> MAARWSSENVVVEFRDSQATAMSVDCLGQHAVLSGRRFLYIVNLDAPFEGHRKISRQSKWDIGAVQWNPHDSFAHYFAASSNQRVDLYKWKDGSGEVGTTLQGHTRVISDLDWAVFEPDLLVTSSVDTYIYIWDIKDTRKPTVALSAVAGASQVKWNKKNANCLATSHDGDVRIWDKRKPSTAVEYLAAHLSKIHGLDWHPDSEHILATSSQDNSVKFWDYRQPRKYLNILPCQVPVWKARYTPFSNGLVTVMVPQLRRENSLLLWNVFDLNTPVHTFVGHDDVVLEFQWRKQKEGSKDYQLVTWSRDQTLRMWRVDSQMQRLCANDILDGVDEFIESISLLPEPEKTLHTEDTDHQHTASHGEEEALKEDPPRNLLEERKSDQLGLPQTLQQEFSLINVQIRNVNVEMDAADRSCTVSVHCSNHRVKMLVKFPAQYPNNAAPSFQFINPTTITSTMKAKLLKILKDTALQKVKRGQSCLEPCLRQLVSCLESFVN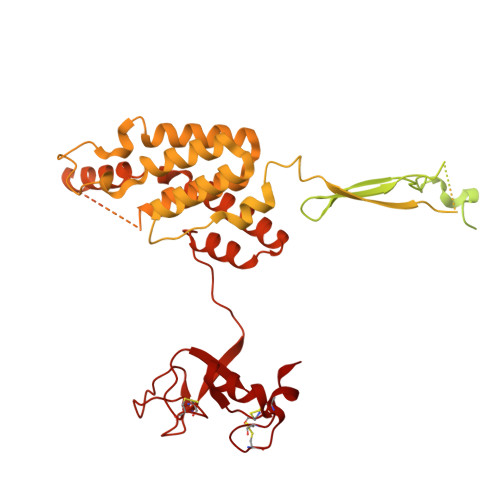QEDSASSNPFALPNSVTPPLPTFARVTTAYGSYQDANIPFPRTSGARFCGAGYLVYFTRPMTMHRAVSPTEPTPRSLSALSAYHTGLIAPMKIRTEAPGNLRLYSGSPTRSEKEQVSISSFYYKERKSRRWKSKREGSDSGNRQIKAAGKVIIQDIACLLPVHKSLGELYILNVNDIQETCQKNAASALLVGRKDLVQVWSLATVATDLCLGPKSDPDLETPWARHPFGRQLLESLLAHYCRLRDVQTLAMLCSVFEAQSRPQGLPNPFGPFPNRSSNLVVSHSRYPSFTSSGSCSSMSDPGLNTGGWNIAGREAEHLSSPWGESSPEELRFGSLTYSDPRERERDQHDKNKRLLDPANTQQFDDFKKCYGEILYRWGLREKRAEVLKFVSCPPDPHKGIEFGVYCSHCRSEVRGTQCAICKGFTFQCAICHVAVRGSSNFCLTCGHGGHTSHMMEWFRTQEVCPTGCGCHCLLESTF> MKLKLIVNGCEAPDDYKLLRTTINTVASLRKTAILRFNSERLTIISTPKSSLNSSNNGTILRGDTGQLWCTIPHDVFRLYTVISARELNTITMECNCDSLLSVFKRYDRVMNQGSSSNMTIKLQSCALGITFEEIVHTSGPNDAIVMNGGVDEHNGLPTTVGTGNLLASNKVIMHSFKVPVKLLFRAQDTRIQEPMINYIQLMMYKLPPISGEFGSAFHGFIRRVERYSNVNHIHLMGVKKKEHGNEGDDVELKIIVNELD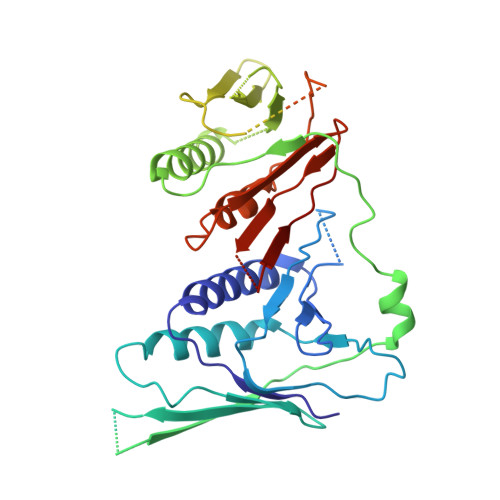WHLEICWNGPLDSVIQRQEGLTDNPSQNQHIDTDGRQEEGSLPIIEADKPMSSLYTNTRDREMEENIRYDEDLLRIEDSSIADTRGNIYTADTSGDTEFNDISVMVEKAEQESSSTHEVIIRCKDWKVCSKLYAAFEEVVLAISHDESCVFHCSLDRGSLEDSEDVEKPRERGQIIYYIARSKGL> SNGLFGANTLSNMGKDTILRFQMFTKWKANGYLPKKIKDDIPRSLYKAYKIHYRMN;> S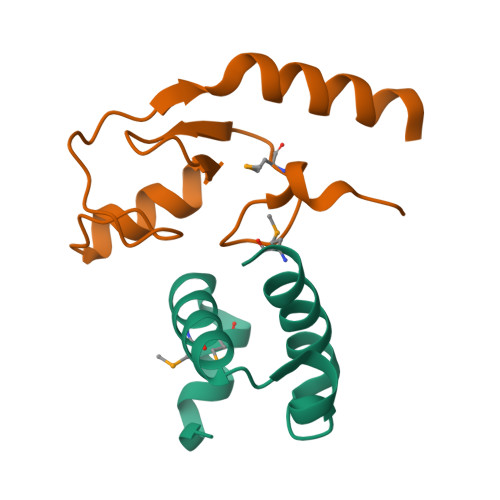HQAPVIPDDFRCPISLELMKDPVIVSTGQTYERTCIEKWLQAGHGTCPKTQQTLTSTVLTPNYVLRSLIAQWCEAN> SGPINDTDANPRYKIPVEADFLFAYSTVPGYYSWRSPGRGEWFVQALCSILEEHGKD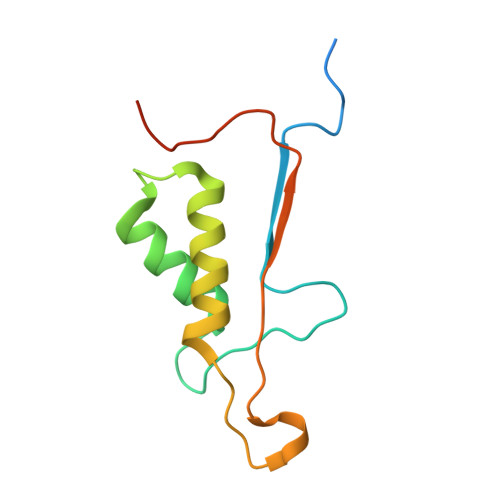LEIMQILTRVNDRVARHFESQSDDPHFHEKKQIPCVVSMLTKELYFSQLEHHHHHH> EAALGDAKDALYAALEGMNRGIFGMTSEKRSEIHALVELLESKNPTPEPTDKLQDKVDGCWRLVYSTISILGKKRTKLGLRDFISLGDFFQMIDVKEEKAVNVIKFSARALKILSGQLTIEASYKITTKTK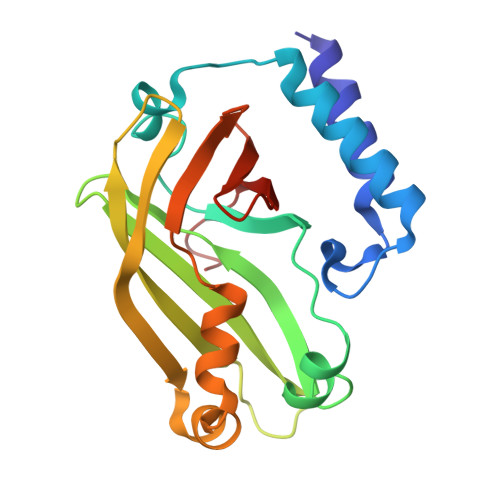VDITLDSSTITPDQLMNIFQKNYDMLLAIFNPEGWLEITYVDESLRIGRDDKANIFVLERADPSEV> MAEPVENKNQAPAPGAKVPPKGAPAAPKAGAPAAPKGPVAPKAGAPAAKTGASAAKQAGKPRLASLGVTLGRSGVRQESALPYVKPKAVPPPKPAAPAAKGAPAPKGAPAAPAAKAAPGAPVAKAAPKAKKHYFIIENLCVGCGLC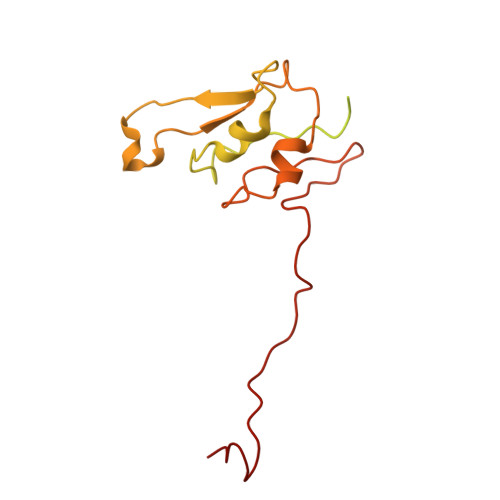LDKCPPKVNAIGYKFYGDVQEGGFRCYIDQAACISCSACFSGDECPSGALIEVLPDGEVLDFSYTPPERLDFDLRFLHRFHREA>[5x]MATERTLSIIKPDAVAKNVIGEIESRFEKAGLKIVAAKMLQLSQEQAEGFYAEHKERPFFGDLVGFMTSGPVVVQVLEGENAIAANRDLMGATNPKEAEAGTIRADYAQSIDANAVHGS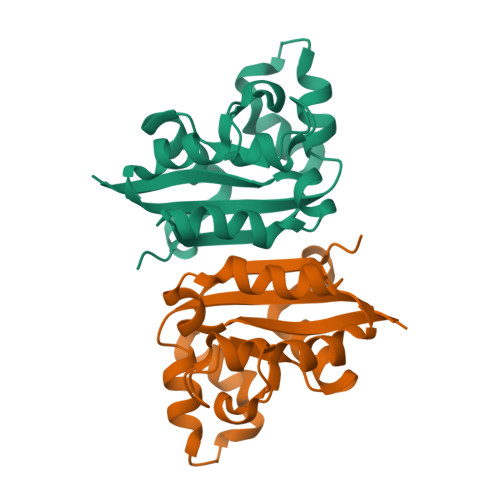DSPESAAREIAYFFEESEICSR>[2x]MFKTEFEFPEELKTKLQEHINYF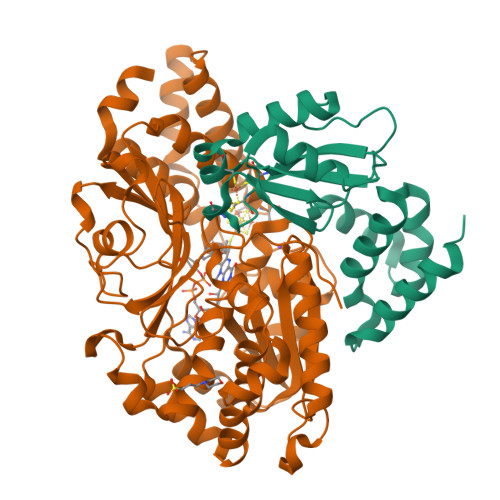PKKRQAILLCLHEIQNYYGYIPPESLKPLADMLELPLNHVEGVVAFYDMFDREDKAKYRIRVCVSIVCHLMGTNKLLKALENILGIKPGEVTPDGKFKIVPVQCLDACSEAPVFMVNDDEYKFESEVQLNEILSRYT;>[2x]MRSYPAIPRIYAETTLNMLLKRAKKPRVHSIDEYLKDGGYQALEKALNMSPEEIIDWVDKSTLRGRGGAGFPTGKKWKFAVQNPGPRYFICNADESEPGTFKDRIIIERDPHLLIEGIIISSYAIGANEAYIYIRGEYPAGYYILRDAIEEAKKKGFLGKNILGSGFDLEIYVARGAGAYICGEETALIESLEGKRGHPRLKPPYPVQKGLWGKPTVVNNVETIANVPFIISMGWEEYRYIGPSDYAGPKLFPVSGKVKKPGVYELPMNTTLREVIFKYAGGTLGNKKVKAVFSGALDCFSSEELDIPMDYSPLGFGGTGTVIVLTEEDDIVEAALKIAEFYEHETCGQCTPCRVGCYEQANLLEKIYKGEATEQDWEGFDFVNRNIQPTSICGLGAVAGRLIRQTLEKFPEEWEKYRKKSASLPLAGHHHHHH> KDDMKAAEQYQGAASAVDPAHVVRTNGAPDMSESEFNEAKQIYFQRCAGCHGVLRKGATGKPLTPDITQQRGQQYLEALITYGTPLGMPNWGSSGELSKEQITLMAKYIQHTPPQPPEWGMPEMRESWKVLVKPEDRPKKQLNDLDLPNLFSVTLRDAGQIALVDGDSKKIVKVIDTGYAVHISRMSASGRYLLVIGRDARIDMIDLWAKEPTKVAEIKIGIEARSVESSKFKGYEDRYTIAGAYWPPQFAIMDGETLEPKQIVSTRGMTVDTQTYHPEPRVAAIIASHEHPEFIVNVKETGKVLLVNY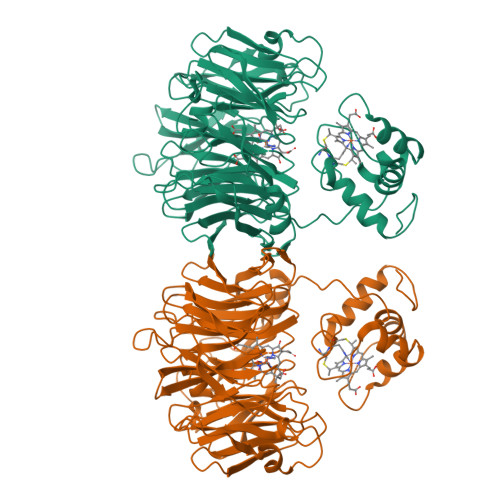KDIDNLTVTSIGAAPFLHDGGWDSSHRYFMTAANNSNKVAVIDSKDRRLSALVDVGKTPAPGRGANFVHPKYGPVWSTSHLGDGSISLIGTDPKNHPQYAWKKVAELQGQGGGSLFIKTHPKSSHLYVDTTFNPDARISQSVAVFDLKNLDAKYQVLPIAEWADLGEGAKRVVQPEYNKRGDEVWFSVWNGKNDSSALVVVDDKTLKLKAVVKDPRLITPTGKFNVYNTQHDVY> MNDNYQNNYVVGRGTVYFDRFQDGTNRKTGEMYFGNTPEFTINTDSETLDHY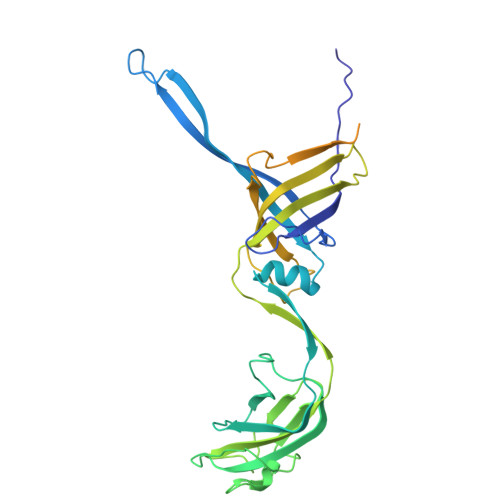SSDHGMRVMDASVLLEASQGGTFTCDNINADNLALWFLGEVSNTTQTQQTDAKEVFNPIMRGRYYQLGTTDDNPTGVRGVTNFQMVKADASIAISVGSGDITSIVGATVVNPAGNYEIDLEAGRIYIEPDSTDLSGNVQIAVQYDVDAQKRTLVIGKSNMVYGALRMISDNPVGLNKNYYFPKVSIAPDGDYALKGDDWQVMSFTFKAMQLNNITQRVYIDIVEAAAAVDPTAQRTIEITPASTTATTGGAGVVCTVTVRDGTGTAVQGDAVTFTTVAGATVTPNSATTGATGTATTTVNRAAAGTATVTATLANGKAATTGTITFSAP>[4x]MIRTGTQYLESLNDGRNVWVGNEKIDNVATHPKTRDYAQRHADFYDLHHRPDLQDVMTYIDEGGQRRAMQWFGHRDKEQLRRKRKYHETVMREMAGASFPRTPDVNNYVLTTYIDDPAPWETQSIGDDGHIKAGKIVDFIRYAREHDLNCAPQFVDPQMDRSNPDAQERSPGLRVVEKNEKGIVVNGVKAIGTGVAFADWIHIGVFFRPGIPGDQVIFAATPVNTPGVTIVCRESLVKDDKVEHPLAAQGDELDGMTVFENVFIPWSHVFHIGNPNHAKLYPQRVFDWLHYHALIRQMVRAELVAGLAVLITEHIGTNKIPAVQTRVAKLIGFHQAMLAHLIASEELGFHTPGGHYKPNILIYDFGRALYLENFSQMIYELVDLSGRSALIFASEDQWNDDKLNGWFERMNNGPVGRPHDRVKIGRVIRDLFL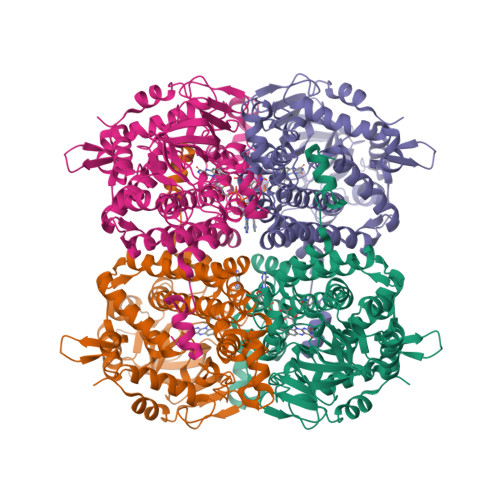TDWGSRLFVFENFNGTPLQGIRMLTMQRAEFSGSGPYGKLARQVCGIDSAVTDDTEYRKTADYAKALDAARHQEEVALAGAMAI> QDAKQIADSLSIPPVKAGAKQLPMPSVSGAQIKLLGADYEQLVNSKGKIAPVISDTPVNVSFKVTKDGKEAVSKDYEIMLQAPQAAQGNPKPRIIPEILQWKGGQGEYKLGNTVTIACPDKELGKLFAADMEDVLGKKVKLVAPGAKADISLSLLKGGNLGREGYRLQIARDGVRLGAAAPTGLFWGTRTLLQMLRQTPGSVPCGTAVDFPRY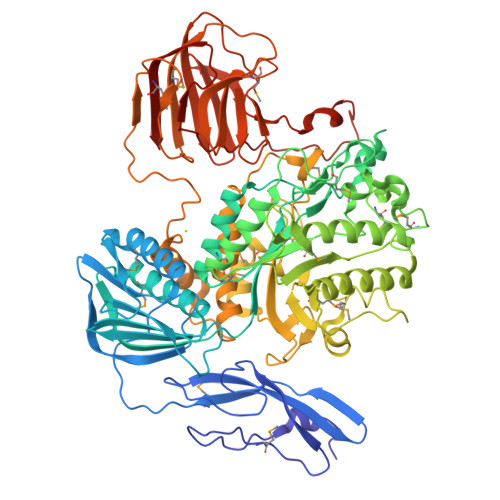QLRGFMLDVARTPYPLSYLKDVIRTMAWYKMNDLHLVINNNYIFHEHYVDNGHDPFKESYAAFRLESKMKGKDGTPLTARDLFYTKKEFADLVSYARKYGVNIVPEFDTPGHALSFTRLRPDLIYKGPMNHEKRRCEMLDAANPETIDLVSKVFDEYMLKDPKLGRPVFADCGVVHVGADEFYGDKEDYRHFANAVLTHALKRGYTPRIWGSLSAKPGKTPVVSKGVQMNLWSTGWMKAWEAVNQGYDVINTNDGALYIVPFAGYYRMDRNHKGLYNNWIPNRIGNETLPSGHPQLLGGTFAVWNDETDIMHTGYAPYDIWGIISGSMDVLSQKLWGTAKAPDTFEQHRELVSSIGNAPRTNPLHKWKDSQPLTVKPSSLPQKLDKPALGPNYRLTMELELTAAPEGKEQVLLAAPEGELLAVMKDGTVGFRRDDSLEFSFGAKLPVGKKVKVEIVGEPEKTSLLLDGEPAGTAVLKNFSDKSKDFSDKFKHRPKVHRSTFILPLKELGSSFQGKVFHMNVQPL;> SIPPVKAGAKQLPMPSVSGAQIKLLGADYEQLVNSKGKIAPVISDTPVNVSFKVTKDGKEAVSKDYEIMLQAPQAAQGNPKPRIIPEILQWKGGQGEYKLGNTVTIACPDKELGKLFAADMEDVLGKKVKLVAPGAKADISLSLLKGGNLGREGYRLQIARDGVRLGAAAPTGLFWGTRTLLQMLRQTPGSVPCGTAVDFPRYQLRGFMLDVARTPYPLSYLKDVIRTMAWYKMNDLHLVINNNYIFHEHYVDNGHDPFKESYAAFRLESKMKGKDGTPLTARDLFYTKKEFADLVSYARKYGVNIVPEFDTPGHALSFTRLRPDLIYKGPMNHEKRRCEMLDAANPETIDLVSKVFDEYMLKDPKLGRPVFADCGVVHVGADEFYGDKEDYRHFANAVLTHALKRGYTPRIWGSLSAKPGKTPVVSKGVQMNLWSTGWMKAWEAVNQGYDVINTNDGALYIVPFAGYYRMDRNHKGLYNNWIPNRIGNETLPSGHPQLLGGTFAVWNDETDIMHTGYAPYDIWGIISGSMDVLSQKLWGTAKAPDTFEQHRELVSSIGNAPRTNPLHKWKDSQPLTVKPSSLPQKLDKPALGPNYRLTMELELTAAPEGKEQVLLAAPEGELLAVMKDGTVGFRRDDSLEFSFGAKLPVGKKVKVEIVGEPEKTSLLLDGEPAGTAVLKNFSDKSKDFSDKFKHRPKVHRSTFILPLKELGSSFQGKVFHMNVQPL;> ADSLSIPPVKAGAKQLPMPSVSGAQIKLLGADYEQLVNSKGKIAPVISDTPVNVSFKVTKDGKEAVSKDYEIMLQAPQAAQGNPKPRIIPEILQWKGGQGEYKLGNTVTIACPDKELGKLFAADMEDVLGKKVKLVAPGAKADISLSLLKGGNLGREGYRLQIARDGVRLGAAAPTGLFWGTRTLLQMLRQTPGSVPCGTAVDFPRYQLRGFMLDVARTPYPLSYLKDVIRTMAWYKMNDLHLVINNNYIFHEHYVDNGHDPFKESYAAFRLESKMKGKDGTPLTARDLFYTKKEFADLVSYARKYGVNIVPEFDTPGHALSFTRLRPDLIYKGPMNHEKRRCEMLDAANPETIDLVSKVFDEYMLKDPKLGRPVFADCGVVHVGADEFYGDKEDYRHFANAVLTHALKRGYTPRIWGSLSAKPGKTPVVSKGVQMNLWSTGWMKAWEAVNQGYDVINTNDGALYIVPFAGYYRMDRNHKGLYNNWIPNRIGNETLPSGHPQLLGGTFAVWNDETDIMHTGYAPYDIWGIISGSMDVLSQKLWGTAKAPDTFEQHRELVSSIGNAPRTNPLHKWKDSQPLTVKPSSLPQKLDKPALGPNYRLTMELELTAAPEGKEQVLLAAPEGELLAVMKDGTVGFRRDDSLEFSFGAKLPVGKKVKVEIVGEPEKTSLLLDGEPAGTAVLKNFSDKSKDFSDKFKHRPKVHRSTFILPLKELGSSFQGKVFHMNVQPL;> KQIADSLSIPPVKAGAKQLPMPSVSGAQIKLLGADYEQLVNSKGKIAPVISDTPVNVSFKVTKDGKEAVSKDYEIMLQAPQAAQGNPKPRIIPEILQWKGGQGEYKLGNTVTIACPDKELGKLFAADMEDVLGKKVKLVAPGAKADISLSLLKGGNLGREGYRLQIARDGVRLGAAAPTGLFWGTRTLLQMLRQTPGSVPCGTAVDFPRYQLRGFMLDVARTPYPLSYLKDVIRTMAWYKMNDLHLVINNNYIFHEHYVDNGHDPFKESYAAFRLESKMKGKDGTPLTARDLFYTKKEFADLVSYARKYGVNIVPEFDTPGHALSFTRLRPDLIYKGPMNHEKRRCEMLDAANPETIDLVSKVFDEYMLKDPKLGRPVFADCGVVHVGADEFYGDKEDYRHFANAVLTHALKRGYTPRIWGSLSAKPGKTPVVSKGVQMNLWSTGWMKAWEAVNQGYDVINTNDGALYIVPFAGYYRMDRNHKGLYNNWIPNRIGNETLPSGHPQLLGGTFAVWNDETDIMHTGYAPYDIWGIISGSMDVLSQKLWGTAKAPDTFEQHRELVSSIGNAPRTNPLHKWKDSQPLTVKPSSLPQKLDKPALGPNYRLTMELELTAAPEGKEQVLLAAPEGELLAVMKDGTVGFRRDDSLEFSFGAKLPVGKKVKVEIVGEPEKTSLLLDGEPAGTAVLKNFSDKSKDFSDKFKHRPKVHRSTFILPLKELGSSFQGKVFHMNVQPL> FKSTTQLIQQVSLTDFFRPDIEHAGST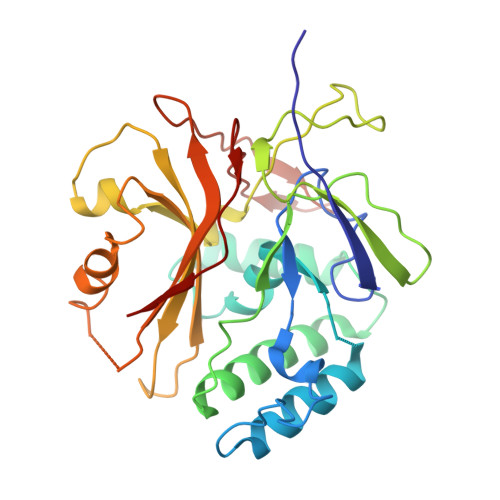VLILRHPTDLPALARHRAPPGRQTERLAEAWGQLLEASRAYVTSLSFIAACRAEEYTDKQAAEANRTAIVSAYGCSRMGARLIRFSECLRAMVQCHVFPHRFISFFGSLLEYTIQDNLCNITAVAKGPQEAARTDKTSTRRVTANIPACVFWDVDKDLHLSADGLKHVFLVFVYTQRRQREGVRLHLALSQLNEQCFGRGIGFLLGARICMYAAYTLIGTIPSESVRYTRRMERFGGYNVPTIWLEGVVWGGTNTWNEC Insulysin (EC 3.4.24.56; also referred to as insulin-degrading enzyme or IDE) is a zinc metallopeptidase in the M16 family that has been extensively studied because of its role in cellular insulin degradation and amyloid beta peptide catabolism. IDE exists predominantly as a dimer in equilibrium with tetramers and to a lesser extent monomers. It is unique among the enzymes comprising the zinc metallopeptidase M16 family in that it exhibits allosteric kinetic behavior with substrate peptides increasing its activity. Crystal structures of human IDE (hIDE) complexed with peptides show that the enzyme consists of four structurally related domains that adopt a clamshell-like structure enclosing a large central chamber.

The E111F mutation greatly reduces catalytic activity while maintaining the ability to bind substrates. Interestingly, though, a difference (Fo-Fc) map made with the rIDE-E111F data in the absence of added substrate peptides revealed two regions of positive electron density located within the central cavity of the enzyme consistent with bound peptide ligand. One segment of difference density was found adjacent to the active site of the enzyme in domain 1, and the second segment was found in the structurally equivalent region of domain 2. The first ligand was modeled as an eight-residue peptide bound at the active site, where it is positioned to interact with the enzyme through a series of hydrogen bonds with the peptide backbone. The second ligand, located at the vestigial active site present in domain 2, the distal site, was modeled as a seven-residue peptide that is also positioned to make a number of hydrogen bond interactions with the enzyme. Both peptides adopt an extended conformation, aligning along the last strand of the central sheet of their respective interacting domains consistent with the usual location of substrate peptides in zinc metallopeptidases. For the peptide in the distal site, the main chain carbonyl groups of Gly339 and Leu359 as well as the side chain of Glu341 are in position to interact with the N-terminal amino group. Additionally, the side chains of Tyr609 and H332 and the main chain carbonyl of Gly361 may make hydrogen bonds with the peptide backbone. Posttranslational modification of this type for polyhistidine fusion sequences of proteins expressed in insect cells has been noted previously. These data indicate that the ligands observed in the crystal structure are the cleaved polyhistidine fusion sequence bound to rIDE-E111F. The conformational change induced by peptide binding seen in this study suggests that allosteric activation occurs by destabilizing the N- and C-terminal domain interface.

> MRNGLVWLLHPALPSTLHSILGARPPPVKRLCGFPKQIYSTMNNPAIQRIEDHIVKSPEDKREYRGLELANGIKVLLISDPTTDKSSAALDVHIGSLSDPPNIPGLSHFCFHMLFLGTKKYPKENEYSQFLSEHAGSSNAFTSGEHTNYYFDVSHEHLEGALDRFAQFFLCPLFDASCKDREVNAVDSEHEKNVMNDAWRLFQLEKATGNPKHPFSKFGTGNKYTLETRPNQEGIDVREELLKFHSTYYSSNLMAICVLGRESLDDLTNLVVKLFSEVENKNVPLPEFPEHPFQEEHLKQLYKIVPIKDIRNLYVTFPIPDLQQYYKSNPGHYLGHLIGHEGPGSLLSELKSKGWVNTLVGGQKEGARGFMFFIINVDLTEEGLLHVEDIILHMFQYIQKLRAEGPQEWVFQECKDLNAVAFRFKDKERPRGYTSKIAGKLHYYPLNGVLTAEYLLEEFRPDLIDMVLDKLRPENVRVAIVSKSFEGKTDRTEQWYGTQYKQEAIPEDVIQKWQNADLNGKFKLPTKNEFIPTNFEILALEKDATPYPALIKDTAMSKLWFKQDDKFFLPKACLNFEFFSPFAYVDPLHCNMAYLYLELLKDSLNEYAYAAELAGLSYDLQNTIYGMYLSVKGYNDKQPILLKKITEKMATFEIDKKRFEIIKEAYMRSLNNFRAEQPHQHAMYYLRLLMTEVAWTKDELKEALDDVTLPRLKAFIPQLLSRLHIEALLHGNITKQAALGVMQMVEDTLIEHAHTKPLLPSQLVRYREVQLPDRGWFVYQRRNEVHNNCGIEIYYQTDMQSTSENMFLELFCQIISEPCFNTLRTKEQLGYIVFSGPRRANGIQGLRFIIQSEKPPHYLESRVEAFLITMEKAIEDMTEEAFQKHIQALAIRRLDKPKKLSAECAKYWGEIISQQYNYDRDNIEVAYLKTLSKDDIIKFYKEMLAVDAPRRHKVSVHVLAREMDSCPVVGEFPSQNDINLSEAPPLPQPEVIHNMTEFKRGLPLFPLVKPHINFMAAKL>[3x]MGITYRDAQIFSACVEALSARNNRITLTSFPLTAGQGQAPTATPAWYPVDLFVADATAVYGRRQLFAWTVDKVRPTRNVAFVTDRVAMDFSAALLSLMAELEAVAPDVYAAIHGGATPGADLGDRITQLENRRVGCLAYVMATVVRAPITHNVRSFSAMLASDPQAHAALLAYLTPNSAGQLDGAPIYFRRSDVDLRNNHLALHAEVVPGLPNMVPLTKAMVEVALANVEWWSDPLGYDSLTSFGGLELLSLCDALAVCELSVAYGLKESGYCYLRFAGGCPLAEVILARLGYNPPLGVAVGWALYNGIKLDWYSKVISVGHNMRLHVCDTAGEANACLIDVLTGEYDGMPVGGVDTVSCWVEQLDLLAAAAGVGRNLSNLHCGVQTPPRTINTTRRRLLASLVRTLIADPTLTDEELLHGAVRGTLNGLPRDRALWRCLQVVNTTVREFLAQDLDAMVRDRRECTTYASRAAFAERCAMSGNASGLVGRQYSDMPAALEGEARACGLSAIDAIEIVRVVASGEPIRVLLDQHGRPATRPNGRLTADELRRCRPLVVGQGGQVGFLPFVPFIVGGVGATVAAASGLALATFATVTGAGAVALGGLGLGAGVAALSITVGQLSYQVTRRALTTILPGGREFGLDDLTRVLGGMVGRYISFVDTWFAHGRGDVFQETDAVPAGTVVFVLPNIEYEVLELRERALGRWSTLLVTTPNGVIAMRANGALPLRVVDAREAGQTFEWSTAARRRFTRAQANAINMMVTASKRVPGLKGSID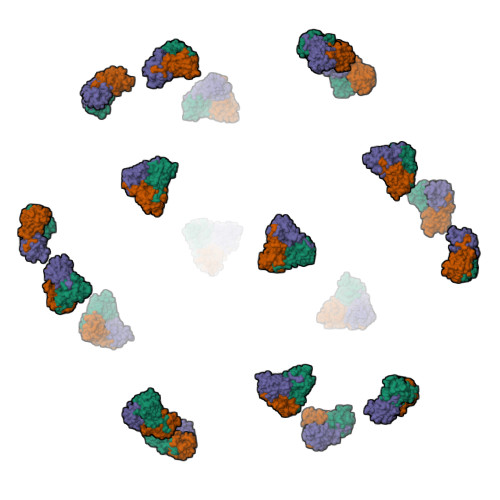AAPSQGTGGSGTDLAGILQRLSALEQTSVPRAEFDALQGRVAACEAKITELEADRVPRIDFTELRDRVHHIDGIGLSCLAHLARDLGITVPHNVRTFRQMRANVGEVIWARFVDAVAESFSPMGGRPIFVRTDPAQPRNNHVSLVDEPTTTGFNGTVTPAMRRLTVADLTGDLVDTEWFSWTPYDASGPLGGTIEGIEAYLTDFTSKLKAELEATPTRTELGVAVGTRAPPLSDRLAAVERVIGMQEGNQVWRSNELRELWVAIDSIVTGRGQREFTTATIKWPAAFPSAVATAGRSFGQPGLAGYGELCTLARQLNALVAGVRNGVVSGMTRNGAGVLQLSTISSATGNLTSDQQAVLRACFFPATPRVGEYQIVYPVGGTMGLTRVDPSTNSSIGQYTRESLVAARNAMPRFAVHTTTPDTVGVAWDNQSAAGLPMGAAPVLTVSVNQLSGVPVTEADKQRWDAKQDKFKIVNTDDRVAALSWVDSVDGFAAPGSDMLLDYQAPAGTGSLPFGSKYAMAVAIGGSLGSQLSEAQVSAARVVLGNGVWRDAVIDVLRKLHNVMYGGKYGRIDDIAAMRSYLNDGTGLLPGSEPIVDVGGAEGNACARATILLRGFSSTMVGVDLKIQMLVELYGAEPATAALLYRGWTMQ> MKILHTSDWHLGVTSWTSSRPVDRREELKKALDKVVEEAEKREVDLILLTGDLLHSRNNPSVVALHDLLDYLKRMMRTAPVVVLPGNQDWKGLKLFGNFVTSISSDI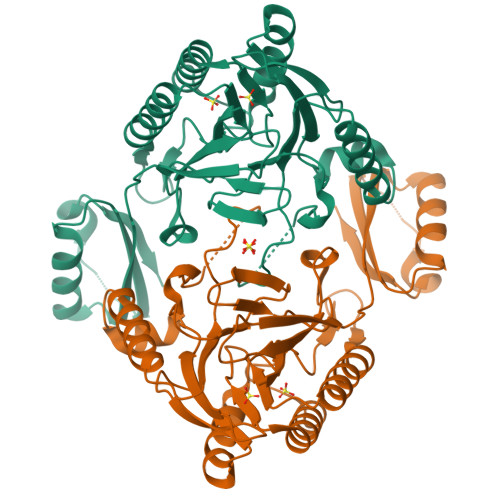TFVMSFEPVDVEAKRGQKVRILPFPYPDESEALRKNEGDFRFFLESRLNKLYEEALKKEDFAIFMGHFTVEGLAGYAGIEQGREIIINRALIPSVVDYAALGHIHSFREIQKQPLTIYPGSLIRIDFGEEADEKGAVFVELKRGEPPRYERIDASPLPLKTLYYKKIDTSALKSIRDSCRNFPGYVRVVYEEDSGILPDLMGEIDNLVKIER>MATAAEIAALPRQKVELVDPPFVHAHSQVAEGGPKVVEFTMVIEEKKIVIDDAGTEVHAMAFNGTVPGPLMVVHQDDYLELTLINPETNTLMHNIDFHAATGALGGGGLTEINPGEKTILRFKATKPGVFVYHCAPPGMVPWHVVSGMNGAIMVLPREGLHDGKGKALTYDKIYYVGEQDFYVPRDENGKYKKYEAPGDAYEDTVKVMRTLTPTHVVFNGAVGALTGDKAMTAAVGEKVLIVHSQANRDTRPHLIGGHGDYVWATGKFNTPPDVDQETWFIPGGAAGAAFYTFQQP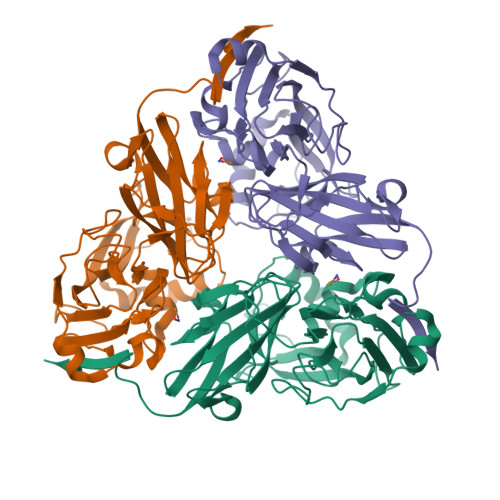GIYAYVNHNLIEAFELGAAAHFKVTGEWNDDLMTSVLAPSGTLVPR[3x]>MALDAAYCFRNVQDNCCLRPLYIDFKRDLGWKWIHEPKGYNANFCAGACPYRASKSPSCVSQDLEPLTILYYIGNTPKIEQL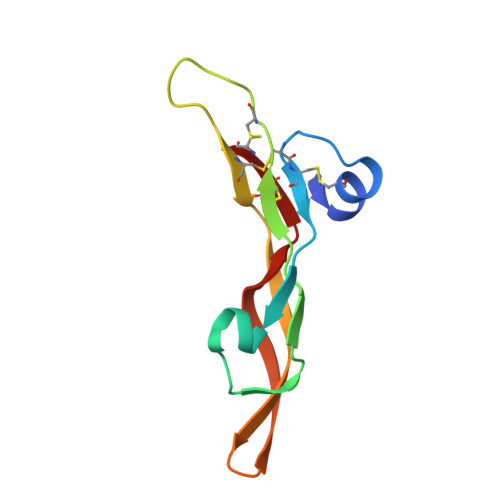SNMIVKSCKCS[2x]>MVDNSRTRPRVGHIQFLNCLPLYWGLARTGTLLDFELTKDTPEKLSEQLVRGDLDIGPVTLVEFLKNADDLVA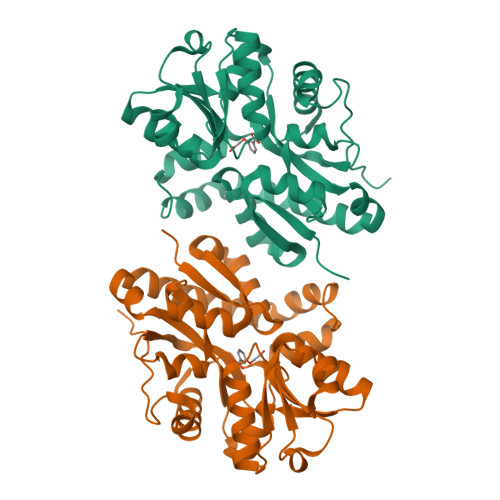FPDIAVGCDGPVMSCVIVSQVPLDRLDGARVALGSTSRTSVRLAQLLLSERFGVQPDYYTCPPDLSLMMQEADAAVLIGDAALRANMIDGPRYGLDVHDLGALWKEWTGLPFVFAVWAARRDYAEREPVITRKVHEAFLASRNLSLEEVEKVAEQAARWEAFDEDTLAKFFTTLDFRFGAPQLEAVTEFARRVGPTTGFPADVKVELLKPLEHHHHHH[2x]>ADSELQLVEQRIRSFPDFPTPGVVFRDISPVLKDPASFRAAIGLLARHLKATHGGRIDYIAGLDSRGFLFGPS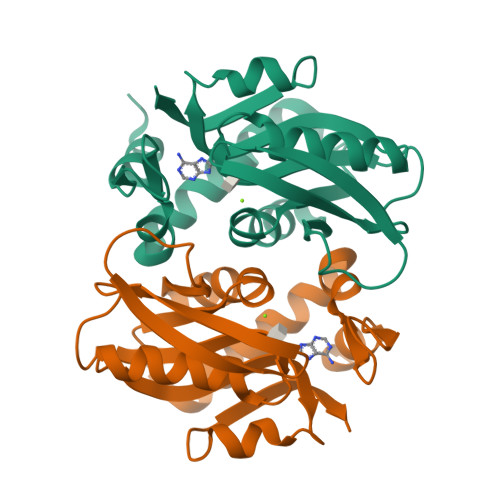LAQELGLGCVLIRKRGKLPGPTLWASYSLEYGKAELEIQKDALEPGQRVVVVDDLLATGGTMNAACELLGRLQAEVLECVSLVELTSLKGREKLAPVPFFSLLQYE[4x]> DLHDKSELTDLALANAYGQYNHPFIKENIKSDEISGEKDLIFRNQGDSGNDLRVKFATADLAQKFKNKNVDIYGASFYYKCEKISENISECLYGGTTLNSEKLAQE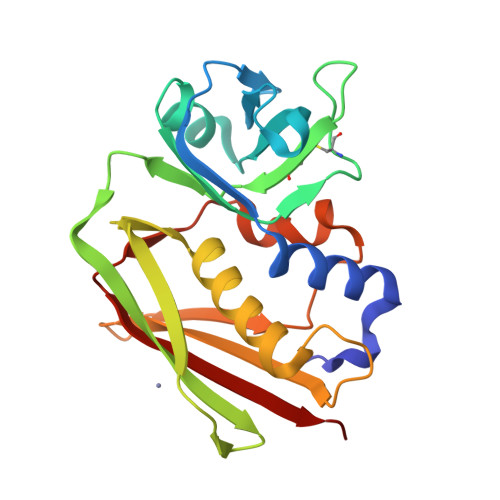RVIGANVWVDGIQKETELIRTNKKNVTLQELDIKIRKILSDKYKIYYKDSEISKGLIEFDMKTPRDYSFDIYDLGGENDYEIDKIYEDNKTLKSDDISHIDVNLYTKK>[2x]SNASTTKLHPLINQKFQS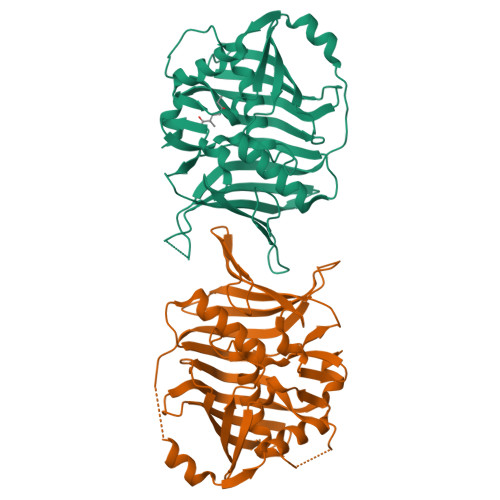PLSKEIFFESYFSTENLPFLADFIVYEQVVVPGASHISLLLAAASLTFAATECQIEDILFPQALAIPEQGVRTVQVVLTPQNNSFSFQVISFDDSLESQINQVSNNGSHISDWAVHATGKLSVANAEQSLIPLEEIQARCSQKIDSAEIYQHLWDRQIHLGQSFRWIEQVWLGEGEVLCQMKVPKTILNTTKYQLHPTLVDSCFQSIIALVLDQSGNKNETFVPFSIDKFTFYNSSDNDLLWCYTCGSKDKQSGEKFKADIQLFDQHGQLVAQVIGFEGRKANPKILLMT[[(2R,3S,5R)-5-[5-(1-benzofuran-2-yl)-2,4-bis(oxidanylidene)pyrimidin-1-yl]-3-oxidanyl-oxolan-2-yl]methoxy-oxidanyl-phosphoryl] phosphono hydrogen phosphate | C17 H19 N2 O15 P3 | 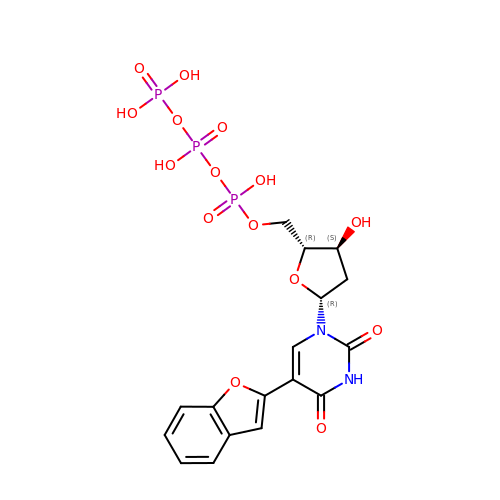VGLLIBLXYZHTBF-NILFDRSVSA-N2-[[(4-chlorophenyl)amino]methyl]-5-propyl-6H-[1,2,4]triazolo[1,5-a]pyrimidin-7-one 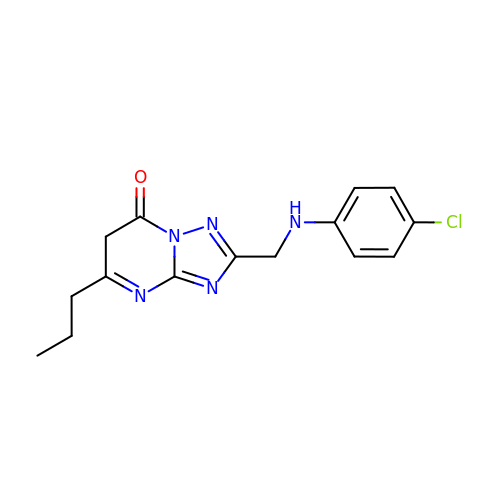| C15 H16 Cl N5 O | FNVJMLMLKHWCHJ-UHFFFAOYSA-N>MAPLENNYNESLNKSKDAIDDKTWSKLFPSIVSDPDRSSNFMIRAIYVVFSAVLRQRNILEKEYFSKNYITENLSCMTLSFKNLRAHQIAQLLRAAGDATKDGFLKEISLVVTEHDGDVEAIEVFSMKFIYFENGGVVARLSTDNNDQEDPHFAELAQLRYEGAESVRDQMVTIVRSVQFLCTKVLEPLPAEFTANFRLKYTNDAPSNFRIDGFDDSSTFYTLPDGIQSVTIGHLRPGHH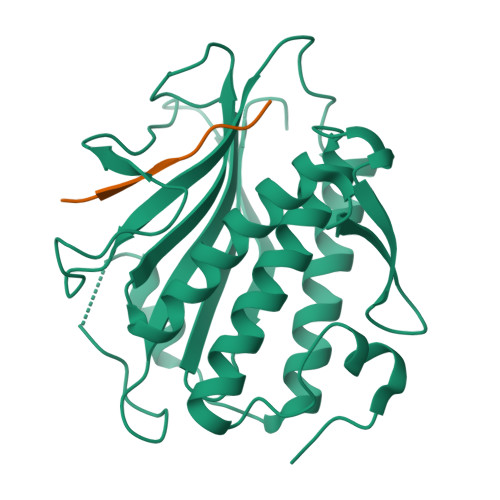AAHMQCWSKSMSD[2x];>[2x]AMRYGQSPNMPSRRGN>GHMEEGIVHKLDVFLIDENVSIKHVNLFDGDSYGCNIHL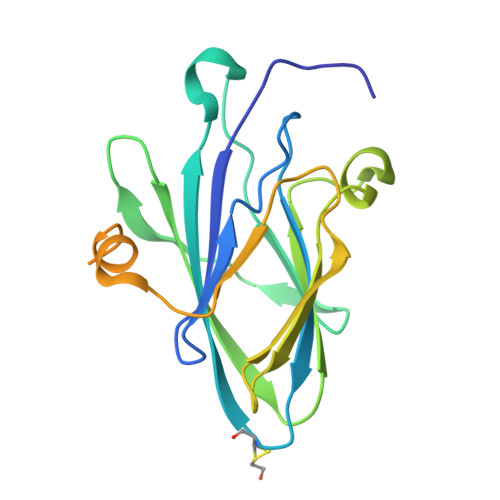KTATCKYITFILVLEPDWENIVEAKPIHMRLNGKKIRVPLVAKTHTSLIYKVVIYVEEDALARFYSDVERSYTDVYPTFLVNTDTRRYYILDSGRTYTYIDPFISDGDKRRWLTREIEEAYDASTEEEEEDDTEEDMDTVHLYCLEEEDEEKIADTGNDNQKDAED[2x]>[2x]MTGPILSGLDPRFERTLYAHVGKEGSWTLDYYLRHGGYETAKRVLKEKTPDEVIEEVKRSGLRGRGGAGFPTGLKWSFMPKDDGKQHYLICNADESEPGSFKDRYILEDVPHLLIEGMILAGYAIRATVGYIYVRGEYRRAADRLEQAIKEARARGYLGKNLFGTDFSFDLHVHRGAGAYICGEETALMNSLEGLRANPRLKPPFPAQSGLWGKPTTINNVETLASVVPIMERGADWFAQMGTEQSKGMKLYQISGPVKRPGVYELPMGTTFRELIYEWAGGPLEPIQAIIPGGSSTPPLPFTEEVLDTPMSYEHLQAKGSMLGTGGVILIPERVSMVDAMWNLTRFYAHESCGKCTPCREGVAGFMVNLFAKIGTGQGEEKDVENLEALLPLIEGRSFCPLADAAVWPVKGSLRHFKDQYLALAREKRPVPRPSLWR;>[2x]MGFFDDKQDFLEETFAKYPPEGRRAAIMPLLRRVQQEEGWIRPERIEEIARLVGTTPTEVMGVASFYSYYQFVPTGKYHLQVCATLSCKLAGAEELWDYLTETLGIGPGEVTPDGLFSVQKVECLGSCHTAPVIQVNDEPYVECVTRARLEALLAGLRAGKRLEEIELPGKCGHHVHEVEV;>[2x]MVRVKVNDRIVEVPPGTSVMDAVFHAGYDVPLFCSEKHLSPIGACRMCLVRIGLPKKGPDGKPLLNEKGEPEIQWQPKLAASCVTAVADGMVVDTLSDVVREAQAGMVEFTLLNHPLDCPTCDKGGACELQDRTVEYGLYEKYYQKGPLELPVYTRFEFTRRHVDKHHPLSPFVILDRERCIHCKRCVRYFEEVPGDEVLDFIERGVHTFIGTMDFGLPSGFSGNITDICPVGALLDLTARFRARNWEMEETPTTCALCPVGCGITADTRSGELLRIRAREVPEVNEIWICDAGRFGHEWADQNRLKTPLVRKEGRLVEATWEEAFLALKEGLKEARGEEVGLYLAHDATLEEGLLASELAKALKTPHLDFQGRTAAPASLFPPASLEDLLQADFALVLGDPTEEAPILHLRLSEFVRDLKPPHRYNHGTPFADLQIKERMPRRTDKMALFAPYRAPLMKWAAIHEVHRPGEEREILLALLGDKEGSEMVAKAKEAWEKAKNPVLILGAGVLQDTVAAERARLLAERKGAKVLAMTPAANARGLEAMGVLPGAKGASWDEPGALYAYYGFVPPEEALKGKRFVVMHLSHLHPLAERYAHVVLPAPTFYEKRGHLVNLEGRVLPLSPAPIENGEAEGALQVLALLAEALGVRPPFRLHLEAQKALKARKVPEAMGRLSFRLKELRPKERKGAFYLRPTMWKAHQAVGKAQEAARAELWAHPETARAEALPEGAQVAVETPFGRVEARVVHREDVPKGHLYLSALGPAAGLRVEGRVLVPAGGEA;>MREEFLEEIPLDAPPEEAKELRTEVMTLNVGPQHPSTHGVLRLMVTLSGEEVLEVVPHIGYLHTGFEKTMEHRTYLQNITYTPRMDYLHSFAHDLAYALAVEKLLGAVVPPRAETIRVI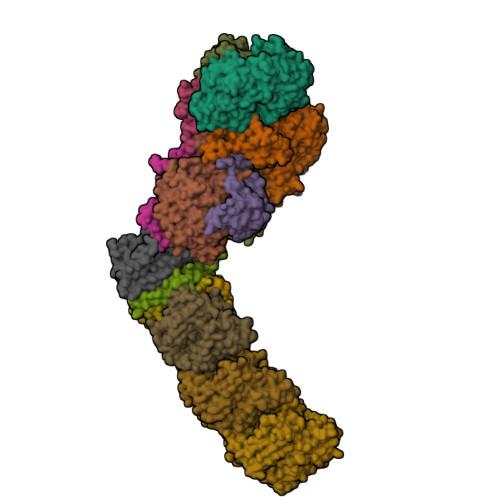LNELSRLASHLVFLGTGLLDLGALTPFFYAFRERETILDLFEWVTGQRFHHNYIRIGGVKEDLPEEFVPELKKLLEVLPHRIDEYEALFAESPIFYERARGVGVIPPEVAIDLGLTGGSLRASGVNYDVRKAYPYSGYETYTFDVPLGERGDVFDRMLVRIREMRESVKIIKQALERLEPGPVRDPNPQITPPPRHLLETSMEAVIYHFKHYTEGFHPPKGEVYVPTESARGELGYYIVSDGGSMPYRVKVRAPSFVNLQSLPYACKGEQVPDMVAIIASLDPVMGDVDR[2x];>[2x]MRLERVLEEARAKGYPIEDNGLGNLWVVLPRERFKEEMAHYKAMGFNFLADIVGLDYLTYPDPRPERFAVVYELVSLPGWKDGDGSRFFVRVYVPEEDPRLPTVTDLWGSANFLEREVYDLFGIVFEGHPDLRKILTPEDLEGHPLRKDYPLGETPTLFREGRYIIPAEFRAALTGKDPGLTFYKGGSRKGYRSLWADLKKAREVKG;>MALKDLFERDVQELEREGILFTTLEKLVAWGRSNSLWPATFGLACCAIEMMASTDARNDLARFGSEVFRASPRQADVMIVAGRLSKKMAPVMRRVWEQMPDPKWVISMGACASSGGMFNNYAIVQNVDSVVPVDVYVPGCPPRPEALIYAVMQLQKKVRGQAYNERGERLPPVAAWKRTRG[2x];>MSASSERELYEAWVELLSWMREYAQAKGVRFEKEADFPDFIYRMERPYDLPTTIMTASLSDGLGEPFLLADVSPRHAKLKRIGLRLPRAHIHLHAHYEPGKGLVTGKIPLTKERFFALADRAREALAFA[2x];>MTLKALAQSLGITLKYLFSKPVTVPYPDAPVALKPRFHGRHVLTRHPNGLEKCIGCSLCAAACPAYAIYVEPAENDPENPVSAGERYAKVYEINMLRCIFCGLCEEACPTGAIVLGYDFEMADYEYSDLVYGKEDMLVDVVGTKPQRREAKRTGKPVKVGYVVPYVRPELEGFKAPTEGGKR[2x];>MAPIQEYVGTLIYVGVALFIGVAALLVGALLGPKKPGRAKLMPYESGNDPAGEVKRFPVHFYVVAMLFILFDVEVAFLWPYAVSAGGLGLYGFLGVLAFTLLLFVGFLYEWWKGVMRWH[2x];>MTWSYPVDPYWMVALKALLVVVGLLTAFAFMTLIERRLLARFQVRMGPNRVGPFGLLQPLADAIKSIFKEDIVVAQADRFLFVLAPLISVVFALLAFGLIPFGPPGSFFGYQPWVINLDLGILYLFAVSELAVYGIFLSGWASGSKYSLLGSLRSSASLISYELGLGLALLAPVLLVGSLNLNDIVNWQKEHGWLFLYAFPAFLVYLIASMAEAARTPFDLPEAEQELVGGYHTEYSSIKWALFQMAEYIHFITASALIPTLFLGGWTMPVLEVPYLWMFLKIAFFLFFFIWIRATWFRLRYDQLLRFGWGFLFPLALLWFLVTALVVALDLPRTYLLYLSALSFLVLLGAVLYTPKPARKGGGA[2x];>[2x]MSLLEGLALFLLLLSGVLVVTLRNAIHAALALILNFLVLAGVYVALDARFLGFIQVIVYAGAIVVLFLFVIMLLFAAQGEIGFDPLVRSRPLAALLALGVAGILAAGLWGLDLAFTQDLKGGLPQALGPLLYGDWLFVLLAVGFLLMAATVVAVALVEPGKASRAKEAEKREEVAR;>MSYLLTSALLFALGVYGVLTRRTAILVFLSIELMLNAANLSLVGFARAYGLDGQVAALMVIAVAAAEVAVGLGLIVAIFRHRESTAVDDLSELRG[2x];>MALLGTILLPLLGFALLGLFGKRMREPLPGVLASGLVLASFLLGAGLLLSGGARFQAEWLPGIPFSLLLDNLSGFMLLIVTGVGFLIHVYAIGYMGGDPGYSRFFAYFNLFIAMMLTLVLADSYPVMFIGWEGVGLASFLLIGFWYKNPQYADSARKAFIVNRIGDLGFMLGMAILWALYGTLSISELKEAMEGPLKNPDLLALAGLLLFLGAVGKSAQIPLMVWLPDAMAGPTPVSALIHAATMVTAGVYLIARSSFLYSVLPDVSYAIAVVGLLTAAYGALSAFGQTDIKKIVAYSTISQLGYMFLAAGVGAYWVALFHVFTHAFFKALLFLASGSVIHALGGEQDVRKMGGLWKHLPQTRWHALIGALALGGLPLLSGFWSKDAILAATLTYPFGGVGFYVGALLVAVLTAMYAMRWFVLVFLGEERGHHHPHEAPPVMLWPNHLLALGSVLAGYLALPHPLPNVLEPFLKPALAEVEAHHLSLGAEWGLIALSAAVALLGLWAGFVFFQRKVFPAWYLAFEAASREAFYVDRAYNALIVNPLKALAEALFYGDRGLLSGYFGLGGAARSLGQGLARLQTGYLRVYALLFVLGALLLLGVMRW[2x];>MVVLAVLLPVVFGALLLLGLPRALGVLGAGLSFLLNLYLFLTHPGGVAHAFQAPLLPGAGVYWAFGLDGLSALFFLTIALTVFLGALVARVEGRFLGLALLMEGLLLGLFAARDLLVFYVFFEAALIPALLMLYLYGGEGRTRALYTFVLFTLVGSLPMLAAVLGARLLSGSPTFLLEDLLAHPLQEEAAFWVFLGFALAFAIKTPLFPLHAWLPPFHQENHPSGLADALGTLYKVGVFAFFRFAIPLAPEGFAQAQGLLLFLAALSALYGAWVAFAAKDFKTLLAYAGLSHMGVAALGVFSGTPEGAMGGLYLLAASGVYTGGLFLLAGRLYERTGTLEIGRYRGLAQSAPGLAALALILFLAMVGLPGLSGFPGEFLTLLGAYKASPWLAALAFLSVIASAAYALTAFQKTFWEEGGSGVKDLAGAEWGFALLSVLALLLMGVFPGYFARGLHPLAEAFAKLLGGGA[2x];>[2x]MTLAILAVFSVALTLLGFVLPPQGVKRATLLGLALALASLLLTWGKPFAFGPYAVDGVSQVFTLLALLGALWTVGLVRSGRFEFYLLVLYAALGMHLLASTRHLLLMLVALEALSLPLYALATWRRGQGLEAALKYFLLGALAAAFFLYGAALFYGATGSLVLGAPGEGPLYALALGLLLVGLGFKAALAPFHFWTPDVYQGSPTPVVLFMATSVKAAAFAALLRVAAPPEALALLVALSVVVGNLAALAQKEAKRLLAYSSIAHAGYMALALYTGNAQALGFYLLTYVLATGLAFAVLSQISPDRVPLEALRGLYRKDPLLGLAFLVAMLSLLGLPPLAGFWGKYLAFAEAARAGAWGVLVLALVTSAVSAYYYLGLGLAVFARPEETPFRPGPPWARAAVVAAGVLLLALGLLPGLVLPALAAGG;>MVRVGMRAAPRVSLEALKAALGGLKLSEAKVYLITDWQDKRDQARYALLLHTGKKDLLVPDAFGPAFPGGEEALSELVGLLLAQGARRFYEAVVSPGEMTALLDLPPEELLKRVMAIANPTDPGIYLKRAA[2x]>[4x]MLLNLDVRMQLKELAQKEFKEPVSIKLFSQAIGCESCQTAEELLKETVEVIGEAVGQDKIKLDIYSPFTHKEETEKYGVDRVPTIVIEGD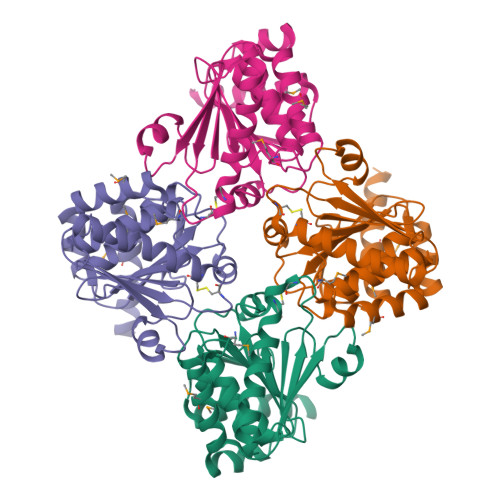KDYGIRYIGLPAGLEFTTLINGIFHVSQRKPQLSEKTLELLQVVDIPIEIWVFVTTSCGYCPSAAVMAWDFALANDYITSKVIDASENQDLAEQFQVVGVPKIVINKGVAEFVGAQPENAFLGYIMAVYEKLKREKEQA> NSDNIFVKPGEDLE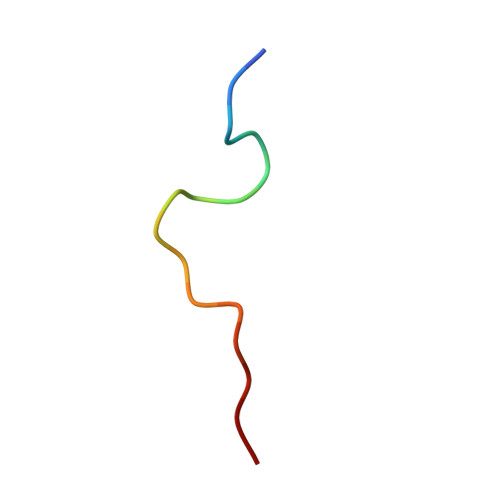IPL>IIGGRESRPHSRPYMAYLQIQSPAGQSRCGGFLVREDFVLTAAHCWGSNINVTLGAHNIQRRENTQQHITARRAIRHPQYNQRTIQNDIMLLQLSRRVRRNRNVNPVALPRAQEGLRPGTLCTVAGWGRVSMRRGTDTLREVQLRVQRDRQCLRIFGSYDPRRQICVGDRRERKAAFKGDSGGPLLCNNVAHGIVSYGKSSGVPPEVFTRVSSFLPWIRTTMR[3x];>IVGGRRARPHAWPFMVSLQLRGGHFCGATLIAPNFVMSAAHCVANVNVRAVRVVLGAHNLSRREPTRQVFAVQRIFENGYDPVNLLNDIVILQLNGSATINANVQVAQLPAQGRRLGNGVQCLAMGWGLLGRNRG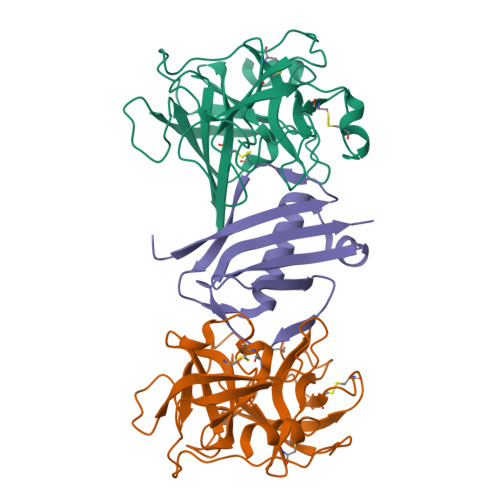IASVLQELNVTVVTSLCRRSNVCTLVRGRQAGVCFGDSGSPLVCNGLIHGIASFVRGGCASGLYPDAFAPVAQFVNWIDSIIQ[3x];>[3x]GSTAEKDKLPATQKAKEMQNVPYTIAVDGIMAFNQSYLNLPKDSQLSYLDLGNKVKALLYDERGVTPEKIRNAKSAVYTITWKDGSKKEVDLKKDSYTANLFDSNSIKQIDINVKTK(2R,3R,4S)-1-[(4-amino-5H-pyrrolo[3,2-d]pyrimidin-7-yl)methyl]-2-(hydroxymethyl)pyrrolidine-3,4-diol 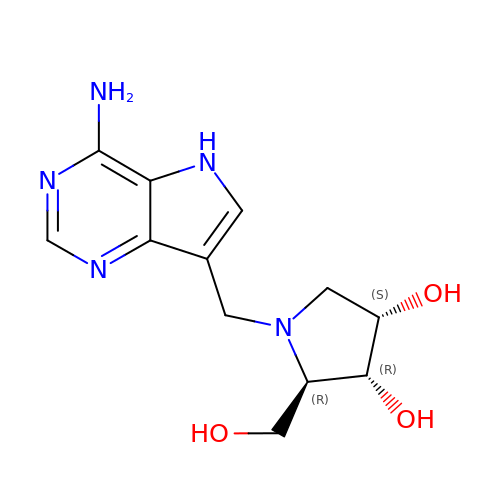| C12 H17 N5 O3 | RCLRGJMFVIDWTM-VHSKPIJISA-N1-[(3-methoxyphenyl)methyl]piperidine-4-carboxamide | C14 H20 N2 O2 | 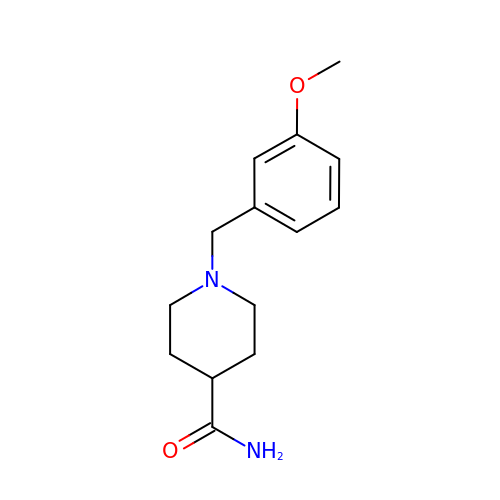WXCVYHZGCBQABJ-UHFFFAOYSA-N2-fluoranyl-5-[2-[(4~{S})-4-methyl-2-oxidanylidene-4-phenyl-pyrrolidin-1-yl]ethoxy]benzenecarbonitrile 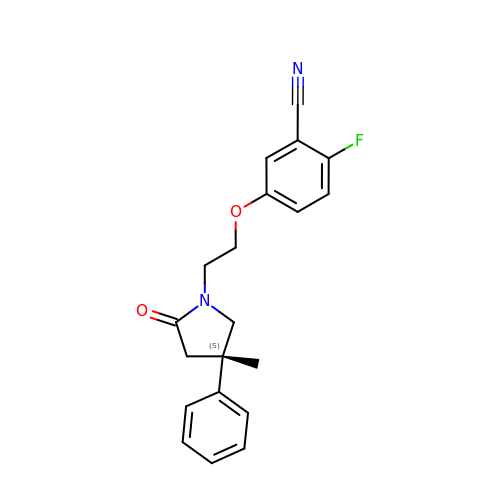| C20 H19 F N2 O2 | WMVNTKWNIVSPIC-HXUWFJFHSA-N> GSMTFPGDTAVLVLAAGPGTRMRSDTPKVLHTLAGRSMLSHVLHAIAKLAPQRLIVVLGHDHQRIAPLVGELADTLGRTIDVALQDRPLGTGHAVLCGLSALPDDYAGNVVVTSGDTPLLDADTLADLIATHRAVSAAVTVLTTTLDDPFGYGRILRTQDHEVMAIVEQTDATPSQREIREVNAGVYAFDIAALRSALSRLSSNNAQQELYLTDVIAILRSDGQTVHASHVDDSALVAGVNNRVQLAELASELNRRVVAAHQLAGVTVVDP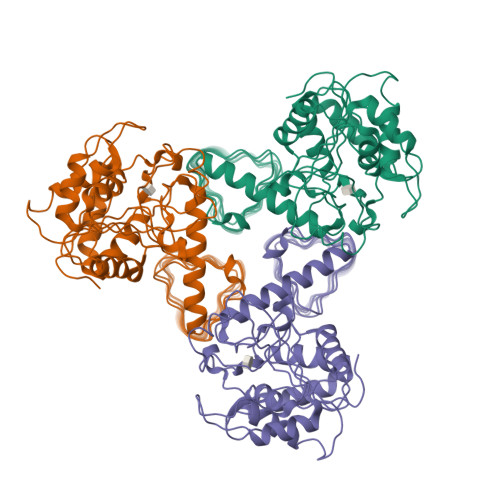ATTWIDVDVTIGRDTVIHPGTQLLGRTQIGGRCVVGPDTTLTDVAVGDGASVVRTHGSSSSIGDGAAVGPFTYLRPGTALGADGKLGAFVEVKNSTIGTGTKVPHLTYVGDADIGEYSNI> GPLGSHHHHHHGGGSGGGSMSFSDQNLIWIDLEMTGLDPEMHKIIEMATIVTDSELNILAEGPVIAIHQPESELAKMDEWCTTTHTASGLVARVRQSQVSEEEAIDQTLAFLKQWVPEGKSPICGNSIGQDRRFLYKHMPRLEAYFHYRYIDVSTIKELTRRWQP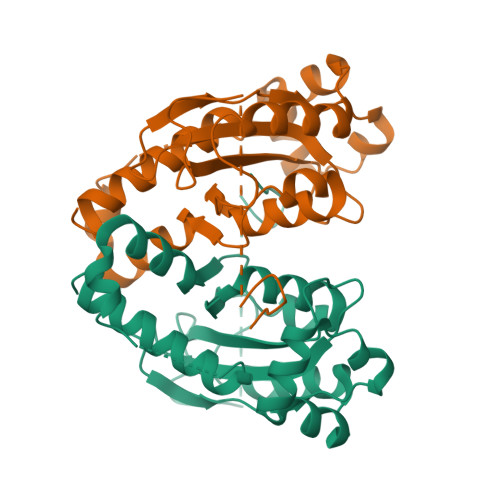EVLKEFSKTGSHLALDDIRESIAELQFYRKAVFKI>GPGMQIKLPKPFFFEEGKRAVLLLHGFTGNSSDVRQLGRFLQKKGYTSYAPQYEGHAAPPDEILKSSPFVWFKDALDGYDYLVEQGYDEIVVAGLSLGGDFALKLSLNRDVKGIVTMCAPMGGKTEGAIYEGFLEYARNFKKYEGKDQETIDNEMDHFKPTETLKELSEALDTIKEQVDEVLDPILVIQAENDNMIDPQSANYIYDHVDSDDKNIKWYSESGHVITIDKEKEQVFEDIYQFLESLDWSE[2x]

Here, we provide the first characterization of S. aureus FphH, a conserved, putative carboxylesterase (referred to as yvaK in Bacillus subtilis) at the molecular and cellular level. Biochemical and structural investigations revealed that FphH acts as an esterase and lipase based on a fold well suited to act on a small to long hydrophobic unbranched lipid group within its substrate and can be inhibited by active site-targeting oxadiazoles. FphH is a member of the α/β hydrolase superfamily illustrated by the well conserved core structure of seven β-strands connected by several helices. The FphH serine hydrolase catalytic triad consists of Ser93, His220, and Asp190 in the usual H-bonding arrangement for this fold to enable the serine residue to cleave substrates that bind to the surrounding active site pockets.

We cloned the full length fphH sequence (SAUSA300_ 0763) using USA300 genomic DNA as a template into a pET28a vector for recombinant expression of the full-length 28 kD enzyme in E. coli, examined behavior in solution, and determined crystallization conditions. FphH crystallized in several different conditions spanning at least three different crystal forms. These crystal forms were very similar and always showed the same monomeric structure, with oligomer analysis in PISA34 also suggesting no oligomer formation in solution. FphH crystals diffracted to higher resolution in the presence of calcium atoms with final models showing Calcium binding on the surface of FphH, especially at crystal contact sites. FphH also contains a well-defined acyl binding pocket that is very hydrophobic, consisting of residues Phe24, Leu94, Pro117, Ile126, Leu168, Met192 and Ile193. In contrast to FphF, FphH is able to accommodate a longer chain in the narrow hydrophobic extension beyond the core acyl binding pocket. The leaving group pocket is not as well-defined, showing a large surface exposed area that is capped about 9 Å away from Ser93 by Asp30. The other sides are defined by the mainchain of Gly23/Gly26 and the side chains of Leu92 and Val221. It is unclear what functional group the leaving group pocket could accommodate from the unbound FphH structure. Helix 125–140 hovers above the active site pockets. The structure suggests that the lid is observed in an intermediate to open state, with Ala125 and Gly129 potentially closing the hydrophobic acyl pocket and Tyr133 interacting with the leaving group in the putative closed state.> MSLRTKGNAELILQIDAYLPDTYISDQRHKIEIYKKIRQIDNRVNYEELQEELIDRFGEYPDVVAYLLEIGLVKSYLDKVFVQRVERKDNKITIQFEKVTQRLFLAQDYFKALSVTNLKAGIAENKGLMELVFDVQNKK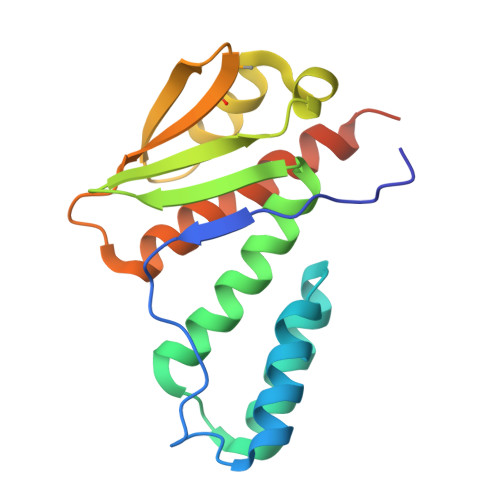DYEILEGLLIFGESLLEIKESKEKNSEGHHHHHH4-[2,4-bis(oxidanylidene)-6-(phenylsulfonyl)-1H-pyrimidin-3-yl]-5-fluoranyl-2-(2-methylphenoxy)benzenecarbonitrile | C24 H16 F N3 O5 S | 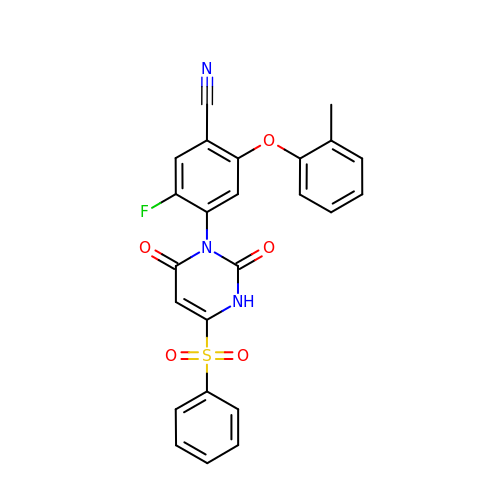UEXYFUXKLNKXPX-UHFFFAOYSA-N Among them one such target is β-clamp. β-clamp, a part of DNA pol III holoenzyme is very crucial protein as it is involved in myriads of steps during DNA replication. It is the key protein that increases the processivity of many important enzymes and complexes by interacting with them. β-clamp prevents the polymerase from dissociating, while polymerase’s rapid movement along the DNA molecule. Biological active form of β-clamp is dimer and each monomeric unit consists of three domains, where the protein-binding site resides in between domain II and III. This interaction site is divided into two subsites and all β-clamp interacting partners bind to these subsites.

All of the five molecules showed competitive binding with ligase and three of them were co-crystallized and determined the complex structure with Hpβ-clamp to show that they bind to the ligase binding site/protein-protein interaction site. In case of (S)-carprofen, Thr154 of Ecβ-clamp makes H-bond with the ligand along with other hydrophobic contacts however in H. pylori the contact between β-clamp and ligand is favored by only hydrophobic interactions. Five of these interactions are common in both, which includes residues Lys151, Thr175, Pro243, Ile248, Met370 in Hpβ-clamp and Arg152, Gly174, Pro242, Val247, Met362 in Ecβ-clamp. Hpβ-clamp residue Thr173 form hydrogen bond with every docked inhibitor, while residue Lys247 hydrogen bonded the docked inhibitors (S)-carprofen. Out of five shortlisted drug molecules 6-Nitroindazole (C2), (S)-Carprofen (C3), and 5-Nitroindole (C4) displayed poor inhibitory activity on the growth of H. pylori, which may have been due to their inability to diffuse into the pathogen.

> MKISVSKNDLENALRYLQAFLDKKDASSIASHIHLEVIKEKLFLKASDSDIGLKSYIFTQSSDKEGVGTINGKKFLDIISCLKDSNIILETKDDSLAIKQNKSSFKLPMFDADEFPEFPVIDPKVSIEVNAPFLVDAFKKIAPVIEQTSHKRELAGILMQFDQKHQTLSVVGTDTKRLSYTQLEKISIHSTEEDISCILPKRALLEILKLFYENFSFKSDGMLAVIENEMHTFFTKLIDGNYPDYQKILPKEYISSFTLGKEEFKESIKLCSSLSSTIKLTLEKNNALFESLDSEHSETAKTSVEIEKGLDIEKAFHLGVNAKFFLEALNALGTTQFVLRCNEPSSPFLIQESLDEKQSHLNAKISTLMMPITL>SRRDFTFDLYRALASAAPSQNIFFSPVSISMSLAMLSLGAGSSTKMQILEGLGLNLQKSSEKELHRGFQQLLQELNQPRDGFQLSLGNALFTDLVVDLQDTFVSAMKTLYLADTFPTNFRDSAGAMKQINDYVAKQTKGKIVDLLKNLDSNAVVIMVNYIFFKAKWETSFNHKGTQEQDFYVTSETVVRVPMMSREDQYHYLLDRNLSCRVVGVPYQGNATALFILPSEGKMQQVENGLSEKTLRKWLKMFKKRQLELYLPKFS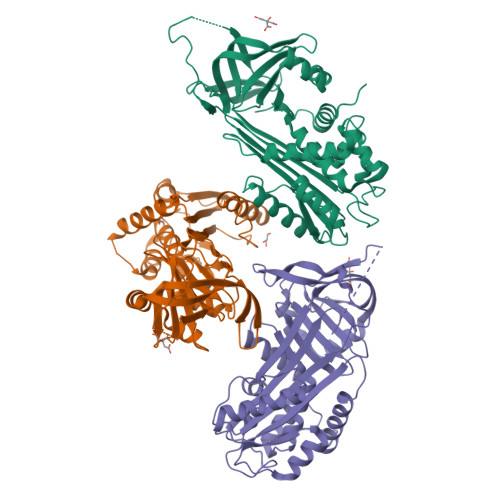IEGSYQLEKVLPSLGISNVFTSHADLSGISNHSNIQVSEMVHKAVVEVDESGTRAAAATGTIFTFRSARLNSQRLVFNRPFLMFIVDNNILFLGKVNRP[3x]>[2x]MFWLKTRIIEGEGSLSRLSREVKGHERVLILASGSMKRHGFLSEAEDYVKEAGAEVFSIAGLPAEPSVEVI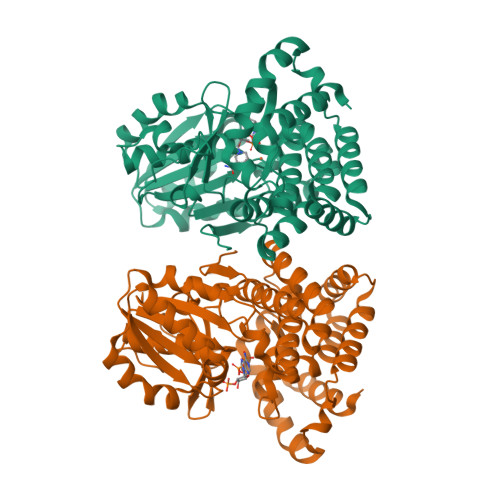EEFLPKVREFGPDLLVAMGGGSVIDTTKALKVFYDAPELNFGEIAFIDRFSKPKPVPRLKTLLIAIPSTSGAGSEVSGASVLKKGGVKYNIVTPEIAPDVAILDPRLPRTMPPEVARNSGLDVLVHGIEAYTTKVASPFSDAMAIKAIKTVYRWLPLSVKGDEEARARVHYAATMAGIAFLNARLGLCHAMSHKAAWIGPHGLLNAVFLPYVMEFNASKSDYARRRYAEIARELGFQTAKDLIEVVKELNEMLGVPKLGELVDEETFASKVEEMAEKTYHDGLIAFNPVEPKPEEIKELYLKAYRGE> MNTISILSTTDLPAAWQIEQRAHAFPWSEKTFFGNQGERYLNLKLTADDRMAAFAITQVVLDEATLFNIAVDPDF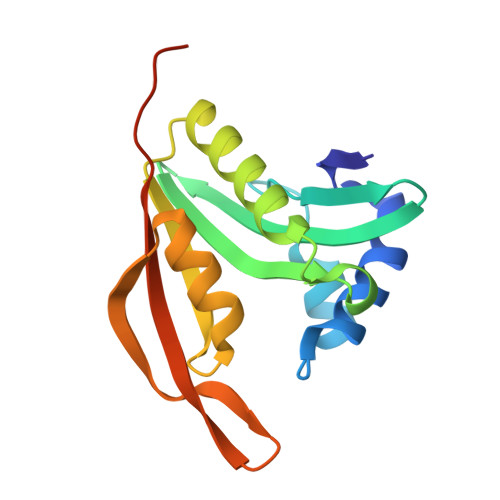QRRGLGRMLLEHLIDELETRGVVTLWLEVRASNAAAIALYESLGFNEATIRRNYYPTAQGHEDAIIMALPISMKLHHHHHHHHHH>[2x]VGLRRRARLSRLVSFSASHRLHSPSLSAEENLKVFGKCNNPNGHGHNYKVVVTIHGEIDPVTGMVMNLTDLKEYMEEAIMKPLDHKNLDL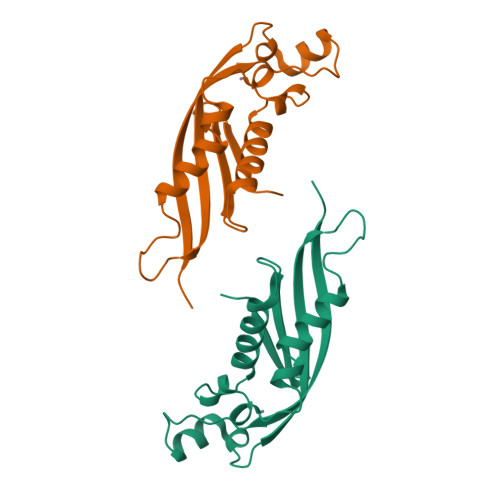DVPYFADVVSTTENVAVYIWENLQRLLPVGALYKVKVYETDNNIVVYKGE> MSAVKKQRIDLRLTDDDKSMIEEAAA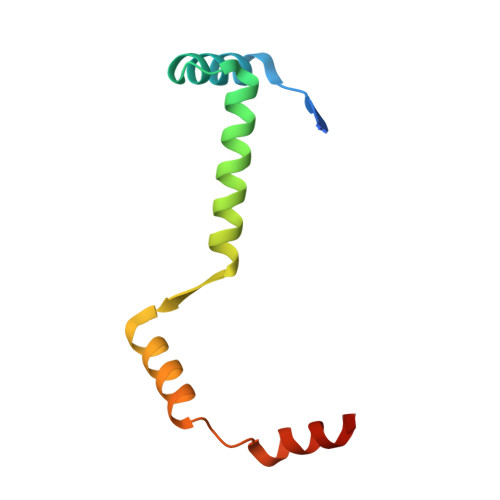ISNQSVSQFMLNSASQRAAEVIEQHRRVILNEESWTRVMDALSNPPSPGEKLKRAAKRLQGM Glutathione, the tri-peptide γ-L-glutamyl-cysteinyl-glycine, is the main low molecular weight thiol antioxidant in both plant and animal cells, often present at millimolar concentrations in vivo. It is synthesised in a two-step, ATP-dependent, process: glutamate-cysteine ligase (GCL) catalyses the formation of γ-glutamylcysteine (γ-EC) from glutamate and cysteine, followed by the addition of glycine by glutathione synthetase (GS) to form glutathione. Cyst nematodes have exploited a series of gene gain events to redeploy glutathione synthetase-like enzymes during parasitism, within the syncytial feeding cell formed in the host root. The most recent expansion has been coupled with a diversification of structure and biochemical function that has given rise to enzymes that are introduced into the host cell, and likely possess novel substrate specificities.

To explore the catalytic capacity of nematode GS-like genes, the G. pallida representative of Clade 1 (Gpa-gss1), one representative from Clade 2 (Gpa-gss5) and a number from Clade 3 (Gpa-gss12, Gpa-gss17, Gpa-gss22, Gpa-gss24 and Gpa-gss30) were heterologously expressed in, and their proteins purified from, bacteria. Remarkably, each stage of the evolutionary process that gave rise to GS-like effectors has witnessed at least a 10-fold reduction in apparent glutathione synthetic rate, such that Clade 3 GS-like proteins have not retained canonical enzyme activity. Comparison between Gpa-GSS22-open and–closed reveals a functioning ATP grasp fold. Residues in the ATP binding pocket of St-GSS1 are highly conserved in sequence and position in the Gpa-GSS22 structure (13/15 residues), and similarly conserved in sequence across G. pallida Clade 3 (structure guided alignment, ~12/15, n = 24). In contrast, there is considerably more variation in the di-peptide binding pocket of G. pallida GS-like effectors, yet, this variation is not evenly distributed around the pocket. However, the glutamate of the di-peptide is exclusively coordinated by interactions with charged side chains of residues in the binding pocket (R, E, 2xQ, N, and Y). All six of these positions are substituted in Gpa-GSS22 and Gpa-GSS30, thus suggesting that the lack of canonical activity is because γ-EC is not accepted despite the potential for cysteine to be accommodated. Variability in the glutamate portion of the di-peptide binding pocket is ubiquitous in G. pallida Clade 3 GS: of the 24 GS-like effectors there are 21 different amino acid compositions in these 6 positions, not one of which is canonical. In summary, conserved amino acids are only absent from one half of the acceptor di-peptide binding pocket. Given that GS effectors have no appreciable rate of ATP turnover when supplied with canonical substrates, yet all display perfect conservation at the catalytic arginine, we infer that GS-like effectors possess a distinct catalytic activity, which may involve alternative substrate(s).

>[4x]MNCDNAKFIIFFFFIIFLCANFAVCNELEDYVEKSVNSETKLHKLADFAIDWAHNNGLILRTKQFLNKSDVAEFAPVSLLPSPFPRHAFEKAVAVHEALQLLYFRVACDYEFMMDAYKDVVNTDNHLRQLVNIIKDAHKQGIKQPTTLLIMRADYMLNTLNSKGNDDEYELKQVEVNTGAIGGLGIDRRTTELHRQMLRKVGMDTSNSPANNGDSNMIESLFMAWEAFGNKNALFVFLSHERLQYKFELRNIQCQLEELSNGQMKVEYVSLKAGYEQLKLGEDYSLLLNGEIVGVVYSTISALGHQANAREMEARRTIELSNAIKAPSLAIAISSSKKIQQLLTTPGTLERFFPSATEADKVAAIRETFTGLWGLEKSDDQTERRIKDAIENPANYVLKSNGECGGNNFYDEALAEKLRTMPQAERASHILMQKLIPMATKNYFLRPFHEPKLNVVVGELGVNGTLLGNLRDQSVRHNVQSGHLLRTKLREANEGGISVGTGVGDSPYLF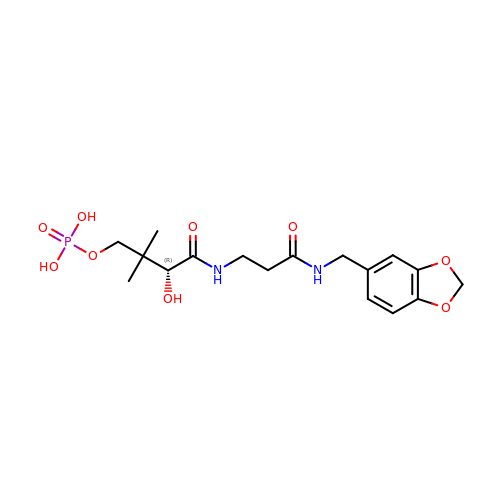N-(1,3-benzodioxol-5-ylmethyl)-N~3~-[(2R)-2-hydroxy-3,3-dimethyl-4-(phosphonooxy)butanoyl]-beta-alaninamide | C17 H25 N2 O9 P | BHYGBZMPSWVNBD-HNNXBMFYSA-N(2S,3S,4R,5R)-2,3,4-TRIHYDROXY-5-HYDROXYMETHYL-PIPERIDINE | 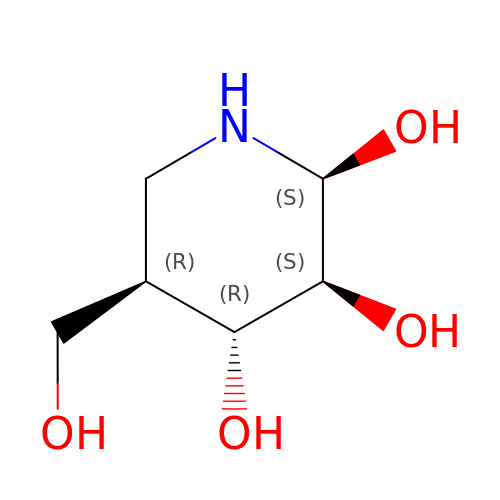C6 H13 N O4 | BHOYFRIRWXBNHP-ZXXMMSQZSA-N> MFARLKRSLLKTKENLGSGFISLFRGKKIDDDLFEELEEQLLIADVGVETTRKIITNLTEGASRKQLRDAEALYGLLKEEMGEILAKVDEPLNVEGKAPFVILMVGVNGVGKTTTIGKLARQFEQQGKSVMLAAGDTFRAAAVEQLQVWGQRNNIPVIAQHTGADSASVIFDAIQ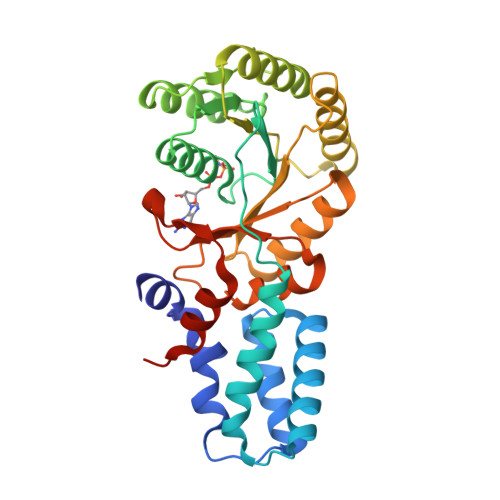AAKARNIDVLIADTAGRLQNKSHLMEELKKIVRVMKKLDVEAPHEVMLTIDASTGQNAVSQAKLFHEAVGLTGITLTKLDGTAKGGVIFSVADQFGIPIRYIGVGERIEDLRPFKADDFIEALFAREDHHHHHH> LLQGFSRWLVFFVSIRIIRHPCRPPYHETYSSSNTFLSIQYIEQSHSARQTSLSLLLITPLTLVLYLAIYTILKMFKTAAAITSLLAASASAFAPSSFNGRISTAVAAEKSQSLPFMNRPPLLDGSMAGDVGFDPLGLSNIDDVGIDLYWLREAEIKHCRVAMLAVVGILQ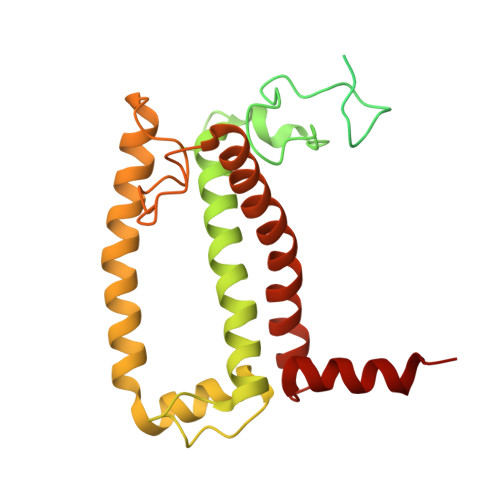VEIFGPAPGCEMATDKCQMDAFWQIWGAHPQYIAFGLIMIMMIEMISGIATTQGRESGERAPGDFGLDPLGYGKGDAAGYARLQAQEIANGRLAMFAAAGEIMQGCTTHQGALENLMTALRDNSF Deltex proteins are a family of E3 ubiquitin ligases that encode C‐terminal RING and DTC domains that mediate interactions with E2 ubiquitin‐conjugating enzymes and recognize ubiquitination substrates. DTX3L has a distinctive domain architecture as it substitutes the WWE domains and proline‐rich region with three domains termed D1, D2 and D3. The N‐terminal D1 and D2 domains of DTX3L mediate homo‐oligomerization, and the D3 domain interacts with PARP9, a protein that contains tandem macrodomains with ADP‐ribose reader function. Our results suggest that homo‐oligomerization of DTX3L is important for the DTX3L‐PARP9 complex to read mono‐ADP‐ribosylation on a ligand‐regulated transcription factor.

Using mass‐spectrometry, we identified that the amino acid sequence of the crystallizable fragment started at A126 and ended in Q200. Taking advantage of the presence of methionine and cysteine residues in the protein sequence we solved the structure by sulfur single‐wavelength anomalous diffraction (S‐SAD) using high‐redundancy data collected on the long‐wavelength beamline I23, at Diamond Light Source, UK. Despite the anisotropy, we observe a well‐defined electron density for the protein, for which we determined that the D2 domain comprises three antiparallel β‐sheets packed against two α‐helices. The asymmetric unit of the crystal had four copies of the D2 monomer, and the interfaces buried in this oligomer (973 and 415 Å2) indicate that this could be a biologically relevant oligomer and that D2 assembles as a homo‐tetramer with a 2‐fold symmetry between adjacent dimers. The larger monomer‐monomer interface corresponds to the head‐to‐head arrangement between the β1 strands of adjacent monomers. This assembly continues the antiparallel β sheet of the monomer with six hydrogen bonds between the strands. At the main interface there is a hydrophobic cleft that accommodates Ile134 and Phe135 from its complementary chain (left). The smaller interface is formed between the short β2 strands and only two inter‐chain hydrogen bonds are formed. Sulfates are located at the N‐terminus of helix α2 and each of them forms a hydrogen bond with H185. Taking all into account, dimer and tetramer are stable in solution, but the structural features suggest that the dimer might be a more stable assembly.

>[4x]AVDSCLQKIFLTVTADLNCNLFSKEQRAYITTLCPSIRKMEGHDGIEKVCGDFQDIERIHQFLSEQFLESEQKQQ5-CHLORO-N-[2-METHOXY-4-[4-(4-METHYLPIPERAZIN-1-YL)PIPERIDIN-1-YL]PHENYL]-N'-(2-PROPAN-2-YLSULFONYLPHENYL)PYRIMIDINE-2,4-DIAMINE | C30 H40 Cl N7 O3 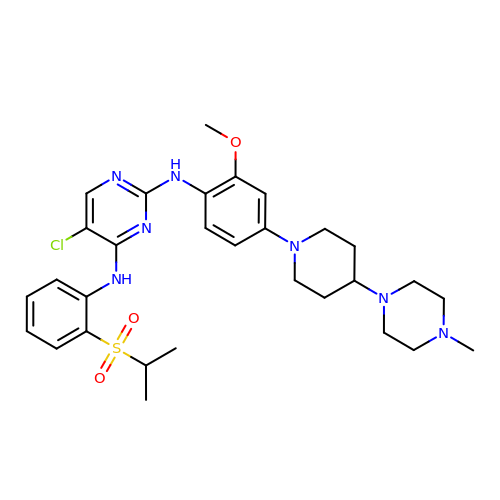S | QQWUGDVOUVUTOY-UHFFFAOYSA-N> MGHHHHHHHHHHGGSENLYFQSGMAFLFSPKARAFSDESLESYLLRVVSENFFDSYEGLSLAIREELHELDFEAHGAFPVDLKRLNVYHAKHNSHFRMRALGLLETLLDLPRYELQKLALLKSDIKFNSSVALYNNGVDIPLRFIRHHAEEAVDSIPVCSQCLAEEAYIKQSWHIKWVNACTKHQCALLHNCPECYAPINYIENESITHCSCGFELSCASTSPVNTLSIEHLNKLLDKGERNDSNPLFNNMTLTERFAALLWYQERYSQTDNFCLNDAVNYFSKWP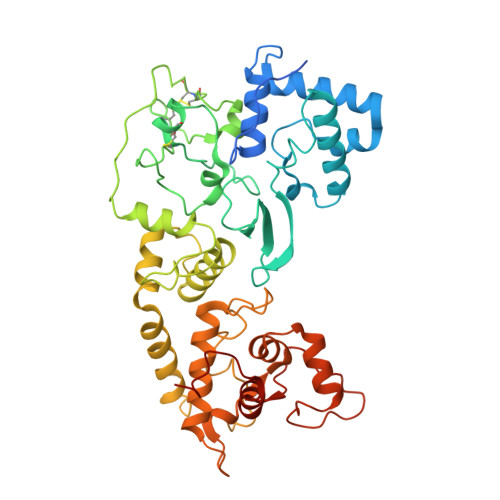AVFNTELDELSKNAEMKLIDLFNKTEFKFIFGDAILACPSTQKQSESHFIYRALLDYLVTLVESNPKTKKPNAADLLVSVLEAATLLGTSVEQVYRLYQNGILQTAFRHKMNQRINPYKGAFFLRHVIEYKTSFGNDKARMYLSAW>[4x]MGF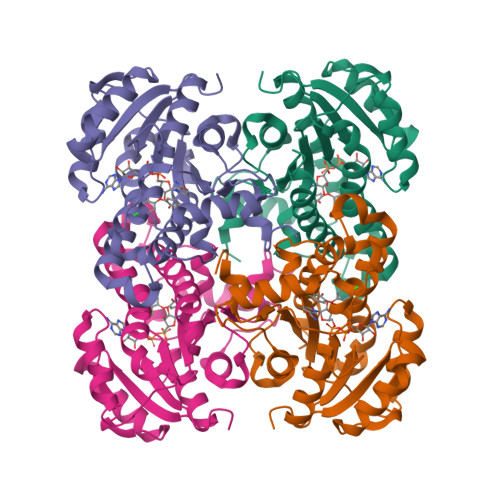LTGKRALIVGVASKLSIASGIAAAMHREGAELAFTYQNDKLRGRVEEFASGWGSRPELCFPCDVADDSQIEAVFAALGKHWDGLDIIVHSVGFAPGDQLDGDFTAVTTREGFRIAHDISAYSFIALAKAGREMMKGRNGSLLTLSYLGAERTMPNYNVMGMAKASLEAGVRYLAGSLGAEGTRVNAVSAGPIRTLAASGIKSFRKMLAANERQTPLRRNVTIEEVGNAGAFLCSDLASGISGEILYVDGGFNTTAMGPLDDDLEHHHHHH> SHMAATAAEAVASGSGEPREEAGALGPAWDESQLRSYSFPTRPIPRLSQSDPRAEELIENEEPVVLTDTNLVYPALKWDLEYLQENIGNGDFSVYSASTHKFLYYDEKKMANFQNFKPRSNREEMKFHEFVEKLQDIQQRGGEERLYLQQTLNDTVGRKIVMDFLGFNWNWINKQQGKRGWGQLTSNLLLIGMEGNVTPAHYDEQQNFFAQIKGYKRCILFPPDQFECLYPYPVHHPCDRQSQVDFDNPDYERFPNFQNVVGYETVVGPGDVLYIPMYWWHHIESLLNGGITITVNFWYKGAPTPKRIEYPLKAHQKVAIMRNIEKMLGEALGNPQEVGPLLNTMIKGRYN

The transcriptional activity of the HIFs is regulated in an oxygen dependent manner by 2-oxoglutarate (2OG) and ferrous iron dependent oxygenases which catalyze the post-translational hydroxylation of HIF-α subunits. Two proline-residues, Pro402 and Pro564 in human HIF-1α, in the N- and C-terminal regions of the oxygen-dependent degradation domains, termed NODD and CODD, respectively, of HIF-α isoforms are efficiently hydroxylated by the HIF prolyl hydroxylases (PHDs or EGLNs) under normoxic conditions. In a second 2OG oxygenase-mediated mechanism of HIF regulation, factor inhibiting HIF (FIH) regulates HIF transcriptional activity via 2OG dependent hydroxylation of an asparagine-residue in the C-terminal transcriptional activation domain (CTAD) of HIF-α isoforms; such reaction reduces binding of HIF to transcriptional co-activator proteins (CBP/p300), which are histone lysine acetyltransferases. Here we report studies that inform on the activities, mechanisms of action, and selectivities of the PHD inhibitors (and related compounds) in clinical trials for anaemia treatment, i.e. Vadadustat from Akebia Therapeutics currently in phase III, FG-4592 from FibroGen in phase III, GSK1278863 from GlaxoSmithKline in phase III, and Molidustat from Bayer in phase II.

The binding mode of GSK1278863 and related compounds (and to a lesser extent, Vadadustat) to 2OG oxygenases is of interest since it has a different scaffold to the FG-2216 related inhibitors. A structure of GSK1278863 (2.45 Å resolution, P41212 space group, 1 molecule per asymmetric unit) with FIH reveals binding to the metal via its amide oxygen (trans to Asp-201), and one ‘pyrimidine-trione’ oxygen (trans to His-279); the GSK1278863 glycinamide carboxylate is positioned to form electrostatic interactions with Lys-214 and Tyr-145. Interestingly, the oxygen of the pyrimidine-trione coordinates the metal trans to the distal histidine, as observed for Molidustat when complexed to FIH. Overlay of the FIH.Zn.GSK1278863 and PHD2.Mn.CCT6 structures reveals an angular difference of 20° (degrees) between the binding mode of the pyrimidone rings of GSK1278863 and CCT6, likely in part due to steric demands of the cyclohexyl rings in GSK1278863. FG-4592, GSK1278863 and Molidustat all manifested no sign of HIF-1α Asn803 hydroxylation inhibition (at least up to 100 μM), consistent with the isolated protein assay results (IC50s for FIH are >100 fold higher than for PHD2). The lack of inhibition of FIH by the clinical PHD inhibitors is also notable (and consistent with cellular results), since the extent to which HIF target genes are regulated by FIH activity (and FIH inhibitors) varies.>[4x]MRGSHHHHHHGSLSSSPSEILQELGKGSTHPQPGVSPPAAPAAPGPKDGPGETDAFGNSEGKELVASGENKIKQGLLPSLEDLLFYTIAEGQEKIPVHKFITALKSTGLRTSDPRLKECMDMLRLTLQTTSDGVMLDKDLFKKCVQSNIVLLTQAFRRKFVIPDFMSFTSHIDELYESAKKQSGGKVADYIPQLAKFSPDLWGVSVCTVDGQRHSTGDTKVPFCLQSCVKPLKYAIAVNDLGTEYVHRYVGKEPSGLRFNKLFLNEDDKPHNPMVNAGAIVVTSLIKQGVNNAEKFDYVMQFLNKMAGNEYVGFSNATFQSERESGDRNFAIGYYLKEKKCFPEGTDMVGIL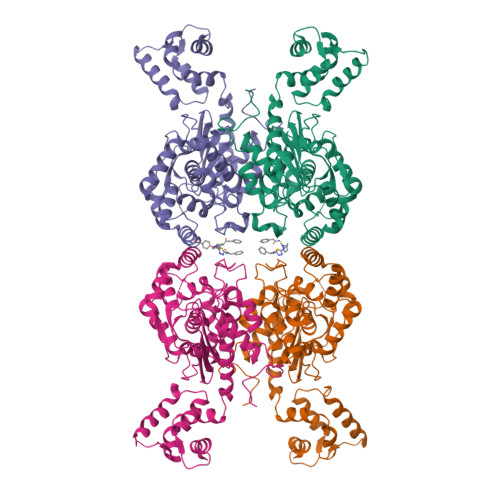DFYFQLCSIEVTCESASVMAATLANGGFCPITGERVLSPEAVRNTLSLMHSCGMYDFSGQFAFHVGLPAKSGVAGGILLVVPNVMGMMCWSPPLDKMGNSVKGIHFCHDLVSLCNFHNYDNLRHFAKKLDPRREGGDQRHSFGPLDYESLQQELALKETVWKKVSPESNEDISTTVVYRMESLGEKS> GQEREAAEYIAQARRQYHFESNQRTCNMTVLSMLPTLREALMQQLNSESLTALLKNRPSNKLEIWEDLKIISFTRSTVAVYSTCMLVVLLRVQLNIIGGYIYLDNAAVGKNGTTILAPPDVQQQYLSSIQHLLGDGLTELITVIKQAVQKVLGSVSLKHSLSLLDLEQKLKEIRNLVEQHKSSSWINKDGSKPLLSHYMMPDEETPLAVQ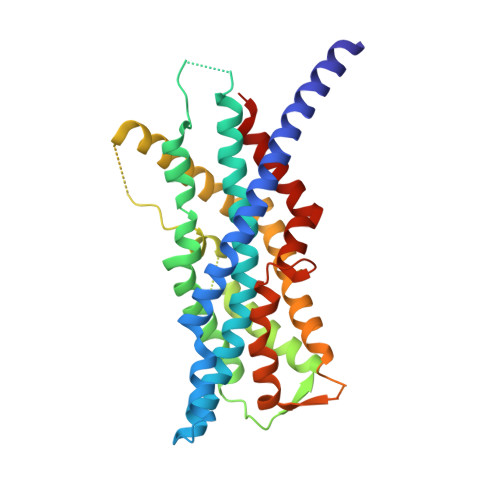ACGLSPRDITTIKLLNETRDMLESPDFSTVLNTCLNRGFSRLLDNMAEFFRPTEQDLQHGNSMNSLSSVSLPLAKIIPIVNGQIHSVCSETPSHFVQDLLTMEQVKDFAANVYEAFSTPQQLEK> HHHHHMPVFHTRTIESILEPVAQQISHLVIMHEEGEVDGKAIPDLTAPVAAVQAAVSNLVRVGKETVQTTEDQILKRDMPPAFIKVENACTKLVQAAQMLQSDPYSVPARDYLIDGSRGILSGTSDLLLTFDEAEVRKIIRVCKGILEYLTVAEVVETMEDLVTYTKNLGPGMTKMAKMIDERQQELTHQEHRVMLVNSMNTVKELLPVLISAMKIFVTTKNSKNQGIEEALKNRNFTVEKMSAEINEIIRVLQLTS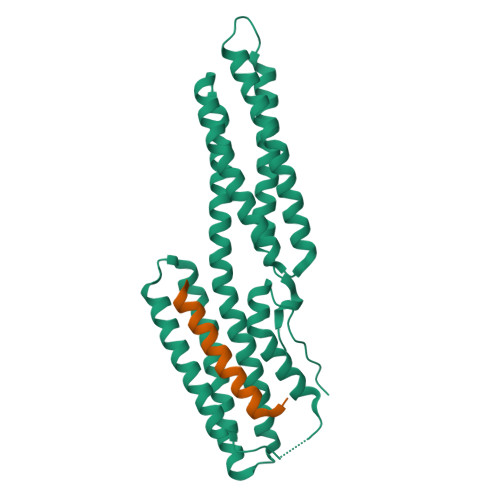WDEDAW;> VGWEQLLTTIARTINEVENQILTR>TTFKIESRIHGNLNGEKFELVGGGVGEEGRLEIEMKTKDKPLAFSPFLLSHCMGYGFYHFASFPKGTKNIYLHAATNGGYTNTRKEIYEDGGILEVNFRYTYEFNKIIGDVECIGHGFPSQSPIFKDTIVKSCPTVDLMLPMSGN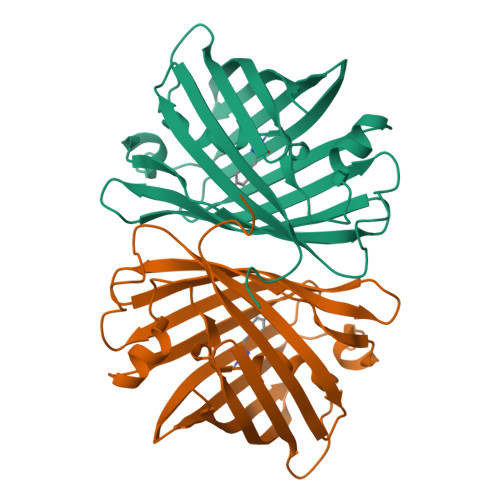IIASSYARAFQLKDGSFYTAEVKNNIDFKNPIHESFSKSGPMFTHRRVEETHTKENLAMVEYQQVFNSAPRDM[2x]>ADEKPDVIDDDIQDEFPDYGFNCEFGWGSHKTFCHWEHDNHVQLKWSVLTSKTGPIQDHTGDGNFIYSQADENQKGKVARLVSPVVYSQNSAHCMTFWYHMSGSHVGTLRVKLRYQKPEEYDQLVWMAIGHQGDHWKEGRVLLHKSLKLYQVIFEGEIGKGNLGGIAVDDISINNHISQEDCAKPAHHHHHH[2x]

Neuropilins (NRPs) are single-pass transmembrane receptors involved in several signaling pathways that regulate key physiological processes such as vascular morphogenesis and axon guidance. Neuropilin-1 (NRP1) and neuropilin-2 (NRP2) exhibit distinct expression patterns; however, they share a common domain organization and 44% amino acid sequence identity in humans (Kolodkin et al., 1997). They are composed of five extracellular structural domains, named a1, at the N terminus, then a2, b1, b2, and c, followed by a single transmembrane helix and a short cytoplasmic tail. The membrane proximal c domain of NRPs is also called the MAM domain (referred to as such in the rest of the text) based on its sequence homology to the equivalent domains in meprin, A5, and mu-phosphatase (RPTPmu) (Takagi et al., 1991, Beckmann and Bork, 1993). Instead, it was proposed that this domain supports dimerization and multimerization of NRP molecules and thus contributes to the formation of signaling receptor complexes (Nakamura et al., 1998).

Here we present the crystal structure of the MAM domain of human NRP1 at 2.24 Å resolution. To overcome this issue all residues that are potential substrates for glycosylation were changed to aspartates to exclude heterogeneity while maintaining negatively charged features of the protein region, thus partially mimicking the effect of glycosylation; this protein variant was named a non-glycosylated MAM (ngMAM) domain. The electron density maps allowed model building for residues 639–813 in chain A and 641–815 in chain B while the N-terminal region (residues 628–639), which contains four of the mutated residues that would be glycosylated in the WT protein, as well as the (His)6 C-terminal tag, was disordered. The crystal structure of the MAM domain of NRP1 comprises a variable N-terminal region that contains a short α helix connected through an extensive linker to a single β strand (βA), and an adjacent eight-stranded β barrel organized in a jellyroll topology, with the strands named B-I, followed by the short α-helical turn at the C terminus. In addition to the polypeptide chain, we were also able to identify two Ca2+ ions and a molecule of bicine associated with each of the NRP1 molecules within the asymmetric unit. The two Ca2+ binding sites are present in both MAM domain molecules within the asymmetric unit and stabilize the domain by bridging the residues from the N-terminal variable region to the first and the last strand of the jellyroll. In contrast to the meprin MAM domain (Arolas et al., 2012), which contains five cysteine residues in the MAM domain of NRP1, no intermolecular disulfide bond can be formed as the four cysteine side chains present form intramolecular disulfide bonds, thus eliminating cysteine-dependent oligomerization as a mechanism of NRP1 self-association.>[2x]GHMSQIPASEQETLVRPKPLLLKLLKSVGAQKD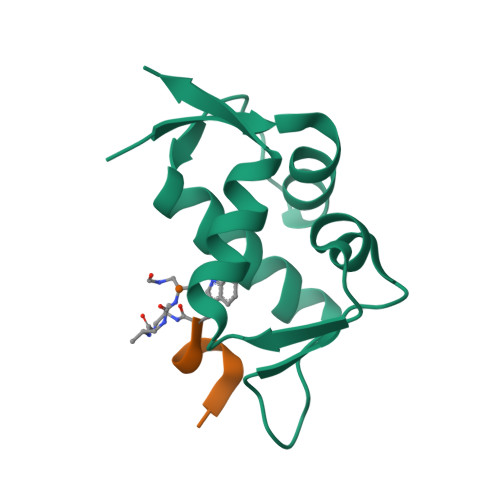TYTMKEVLFYLGQYIMTKRLYDEKQQHIVYCSNDLLGDLFGAPSFSVKEHRKIYTMIYRNLVVVN> MKVLFVSIGNTCRSPMAEAILKHLVVKRNLQDWYVDSAGLRSWNVGLEPQARGQQLLKQHGLKTNHLGRMISAQDFYDFDYIFAMDNSNLLELEHMAASLTPSPTCKIQLLGSYIGRKEDEIIEDPYFIQG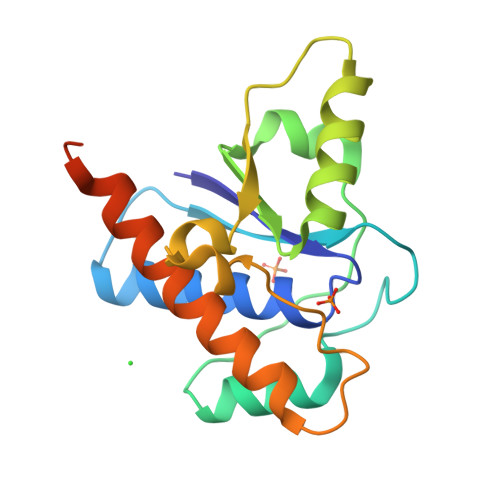MGGFNAAYLQILESCERFLQHYKSDDKELSLGSLEHHHHHH> MGCDAIQAAAALGEAGISSNEILELLAAAAELGLDPDAIQA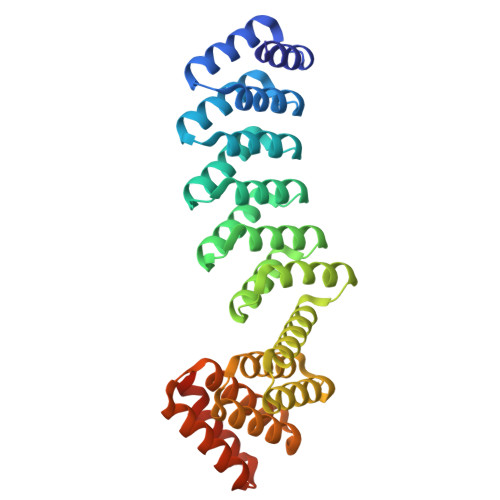AAQLGEAGISSEEIKELLRAAHELGLDPDAIAAAADLGQAGVSPVEILALLIAASVLGLDPDAIQAAAALGEAGISAEEIIELLTAARDLGLDPDAIQAAAQLGEAGISSEEIKELLRAAHELGLDPDCIAAAADLGQAGISSSEITALLLAAAAIELAKRADDKDVREIVRDALELASRSTNDEVIRLALEAAVLAARSTDSDVLEIVKDALELAKQSTNEEVIKLALKAAVLAAKSTDEEVLEEVKEALRRAKESTDEEEIKEELRKAVEEAEGGSWLEHHHHHH> PVFTQDVFVGSVEELSAAHTLVMKINATDAEPNTLSKISYRIVSLEPAYPPVFYLNKDTGEIYTTSV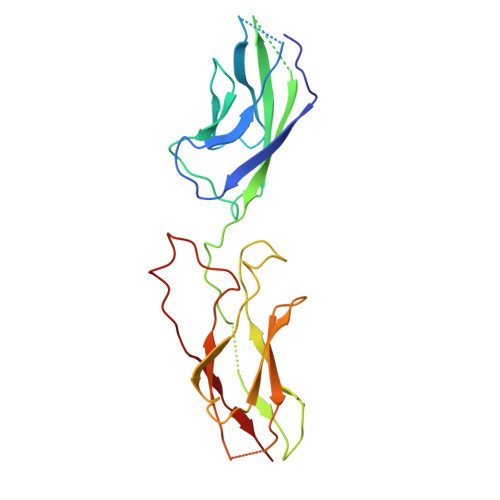TLDREEHSSYTLTVEARDGVKQAQVQIRILDVNDNIPVVELEGMVEENQVNVEVTRIKVFDADEIGSDNWLANFTFASGNEGGYFHIETDAQTNEGIVTLIKEVYMKNLDFSVIVANKAAFHKSIRSKYKPTPIPIKVKVK> MGYVGIKIRLTDVAPQAQELFKKESLDVKENKVYLVAATLRPETMYGQTCCFVSPKIDYGVFDAGNGDYFITTERAFKNMSFQNLTPKRGYYK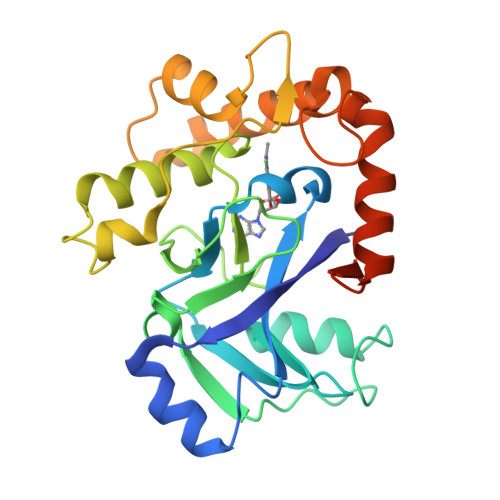PLFTINGKTLIGSRIDAPYAVNKNLRVLPMETVLATKGTGVVTCVPSDSPDDFVTTRDLANKPEYYGIEKDWVQTDIVPIVHTEKYGDKCAEFLVNDLKIQSPKDSVQLANAKELAYKEGFYNGTMLIGKYKGDKVEDAKPKVKQDLIDEGLAFVYNEPELEHHHHHH>MEGAKPTLQLVYQAVQALYHDPDPSGKERASFWLGELQRSVHAWEISDQLLQIRQDVESCYFAAQTMKMKIQTSFYELPTDSHASLRDSLLTHIQNLKDLSPVIVTQLALAIADLALQMPSWKGCVQTLVEKYSNDVTSLPFLLEILTVLPEEVHSRSLRIGANRRTEIIEDLAFYSSTVVSLLMTCVEKAGTDEKMLMKVFRCLGSWFNLGVLDSNFMANNKLLALLFEVLQQDKTSSNLHEAASDCVCSALYAIENVETNLPLAMQLFQGVLTLETAYHMAVAREDLDKVLNYCRIFTELCETFLEKIVCTPGQGLGDLRTLELLLICAGHPQYEVVEISFNFWYRLGEHLYKTNDEVIHGIFKAYIQRLLHALARHCQLEPDHEGVPEETDDFGEFRMRVSDLVKDLIFLIGSMECFAQLYSTLKEGNPPWEVTEAVLFIMAAIAKSVDPENNPTLVEVLEGVVRLPETVHTAVRYTSIELVGEMSEVVDRNPQFLDPVLGYLMKGLAEKPLASAAAKAIHNICSVCRDHMAQHFNGLLEIARSLDSFLLSPEAAVGLLKGTALVLARLPLDKITECLSELCSVQVMALKKLLSQEPSNGISSDPTVFLDRLAVIFRHTNPIVENGQTHPCQKVIQEIWPVLSETLNKHRADNRIVERCCRCLRFAVRCVGKGSAALLQPLVTQMVNVYHVHQHSCFLYLGSILVDEYGMEEGCRQGLLDMLQALCIPTFQLLEQQNGLQNHPDTVDDLFRLATRFIQRSPVTLLRSQVVIPILQWAIASTTLDHRDANCS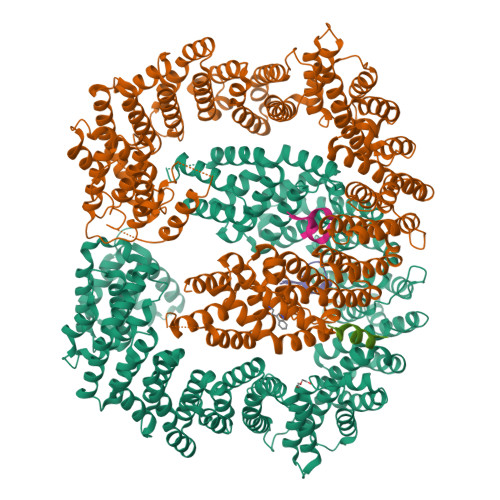VMRFLRDLIHTGVANDHEEDFELRKELIGQVMNQLGQQLVSQLLHTCCFCLPPYTLPDVAEVLWEIMQVDRPTFCRWLENSLKGLPKETTVGAVTVTHKQLTDFHKQVTSAEECKQVCWALRDFTRLFR[2x];>[3x]SRDYYSSRSQSGGYSDRSSGGSYRDSYDSYATHNE>MSLETDDQYYRAIKKIKEAAEASNRAYLTSSKLADMLGISQQSASRIIIDLEKNGYITRTVTKRGQILNITEKGLDVLYTEFADLSRILAIKNNVVITGTVTSGMGEGRYYVARKQYIIQFQEKLGIIPYLGTLNIKVDQA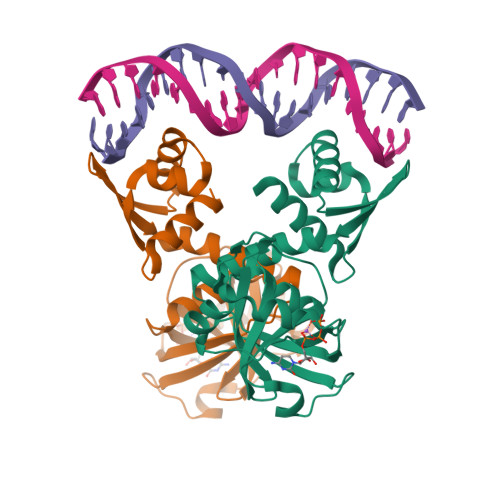SLPELRKIRGFRGIHIEGFKTEDRTFGSVKAFPAKIQNIPCFVIMPERTVYTDVIEIISDKYLREEINLHDGDRVSVEVYTEGHHHHHH[2x]> GNEKLIALTFDDGPSSTTSDVLDILERYGVKATFFLIGQNV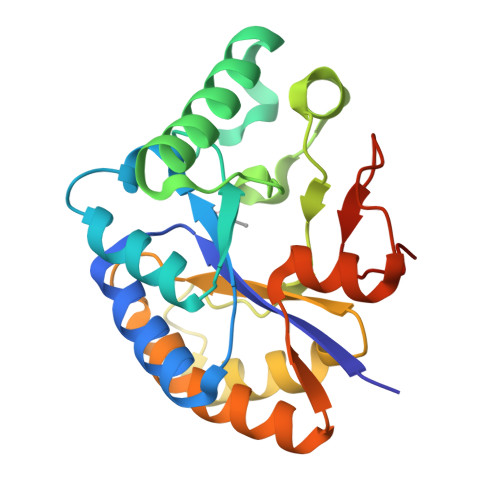NSNTLSIMQRQVRMGCELASHSYTHQDMTNMSAQNIRNEMEWTSSAIKNSVGVDVKFFRPPYIAVNNTMYQNIDYPFIQGTLINDSENSTSVQQRVNNALGAAKDGQIILLHDFQGNSQTVQALPQIIEGLKNQGYTFVTVSELFEKKGVNPNVEYKIWSNANGQHHHHHH>MRPERLTVRNFLGLKNVDIEFQSGITVVEGPNGAGKSSLFEAISFALFGNGIRYPNSYDYVNRNAVDGTARLVFQFERGGKRYEIIREINALQRKHNAKLSEILENGKKAAIAAKPTSVKQEVEKILGIEHRTFIRTVFLPQGEIDKLLISPPSEITEIISDVFQSKETLEKLEKLLKEKMKKLENEISSGGAGGAGGSLEKKLKEMSDEYNNLDLLRKYLFDKSNFSRYFTGRVLEAVLKRTKAYLDILTNGRFDIDFDDEKGGFIIKDWGIERPARGLSGGERALISISLAMSLAEVASGRLDAFFIDEGFSSLDTENKEKIASVLKELERLNKVI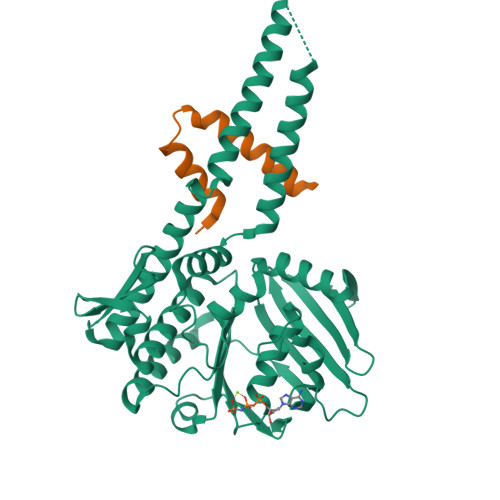VFITHDREFSEAFDRKLRITGGVVVNE[2x];>[2x]KEELDKLDYFELFKEYLKKREENHEKLLKILDELLDEVKKSEAGHHHHHH> SGGSGAGGGELFATHCAGCHPQGGNTVHPEKTLARARREAN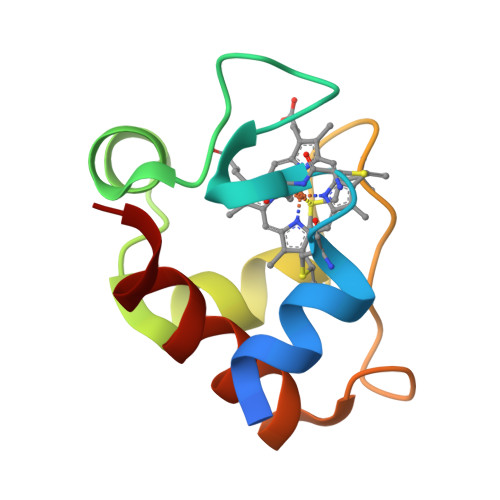GIRTVRDVAAYIRNPGPGMPAFGEAMIPPADALKIGEYVVASFP> GAMESKKRQWALEDF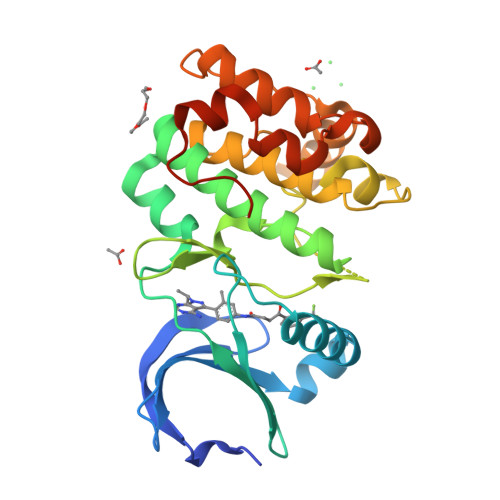EIGRPLGKGKFGNVYLAREKQSKFILALKVLFKAQLEKAGVEHQLRREVEIQSHLRHPNILRLYGYFHDATRVYLICEYAPLGTVYRELQKLSKFDEQRTATYITELANALSYCHSKRVIHRDIKPENLLLGSAGELKIADFGWSVHAPSSRRTTLAGTLDYLPPEMIEGRMHDEKVDLWSLGVLCYEFLVGKPPFEANTYQETYKRISRVEFTFPDFVTEGARDLISRLLKHNPSQRPMLREVLEHPWITANSSKPSNAQNKESASKQS> MPKLVTWMNNQRVGELTKLANGAHTFKYAPEWLASRYARPLSLSLPLQRGNITSDAVFNFFDNLLPDSPIVRDRIVKRYHAKSRQPFDLLSEIGRDSVGAVTLIPEDETVTHPIMAWEKLTEARLEEVLTAYKADIPLGMIREENDFRISVAGAQEKTALLRIGNDWCIPKGITPTTHIIKLPIGEIRQPNATLDLSQSVDNEYYCLLLAKELGLNVPDAEIIKAGNVRALAVERFDRRWNAERTVLLRLPQEDMCQTFGLPSSVKYESDGGPGIARIMAFLMGSSEALKDRYDFMKFQVFQWLIGATQGHAKNFSVFIQAGGSYRLTPFYDIISAFPVLGGTGIHISDLKLAMGLNASKGKKTAIDKIYPRHFLATAKVLRFPEVQMHEILSDFARMIPAALDNVKTSLPTDFPENVVTAVESNVLRLHGRLSREYGSK;> 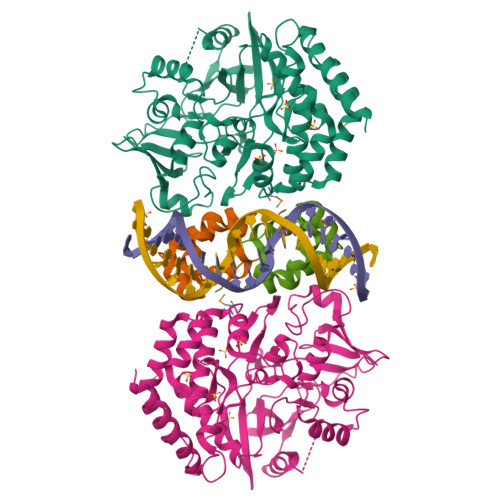MMSFQKIYSPTQLANAMKLVRQQNGWTQSELAKKIGIKQATISNFENNPDNTTLTTFFKILQSLELSMTLCDAKNASPESTEQQNLEW> GCGGAAGUAGUUCAGUGGUAGAACACCCGACAGACGAAGCGCUAAAACGUGGGAUUCUGUCGGGGGGUCGCGGGUUCGAGUCCCGUCUUCCGCUCCA

Bacillus subtilis phage phi29 assembles the genome into a preformed protein capsid (prohead) to near-crystalline density by a highly efficient molecular motor (1–3). The phi29 motor core contains a ribonucleoprotein (RNP) complex of prohead RNA (pRNA) and gene product 16 (gp16) ATPase. This RNP complex actively transports DNA inside the prohead capsid using energy derived from ATP binding and hydrolysis. Phylogenetic analysis and nuclease digestion studies demonstrated that the phi29 pRNA contains two conserved domains: an 120-base domain I and a 54-base Domain II.

The phi29 pRNA domain II-tRNA crystal structure was solved at 3.3 Å resolution using molecular replacement and multiple rounds of fitting. The crystallization construct contains 31 nucleotides of 3′-domain II, a shortened PB helix and the whole PF helix. The secondary structure of pRNA domain II contains two Watson–Crick-paired helices (PF and PB) and two loop regions (LF and LBF). The pRNA domain II crystal structure shows two double RNA helices (PF and PB) connected by a flexible helical turn (LBF). The top helix PF is capped by loop LF. A second possible flexible region, LBF, facilitates a 63-degree turn of the main helix. O2′ of G142 makes an H-bond with N1 of A160 while C141 forms a Watson–Crick basepair with G159, bending the phosphate backbone by ∼60 degrees. Consequently, U161 flips out to accommodate the turn. A160 and U161 display the highest temperature factors due to their flexibility.>[2x]SNAMAIHNRAGQPAQQSDLINVAQLTAQYYVLKPEAGNAEHAVKFGTSGHRGSAGRHSFNEPHILAIAQAIAEERAKNGITGPCYVGKDTHALSEPAFISVLEVLAANGVDVIVQENNGFTPTPAVSNAILVHNKKGGPLADGIVITPSHNPPEDGGIKYNPPNGGPADTNVTKVVEDRANALLAGGLQGVKRISLDAAMASGHVKAVDLVQPFVEGLADIVDMAAIQKAGLTLG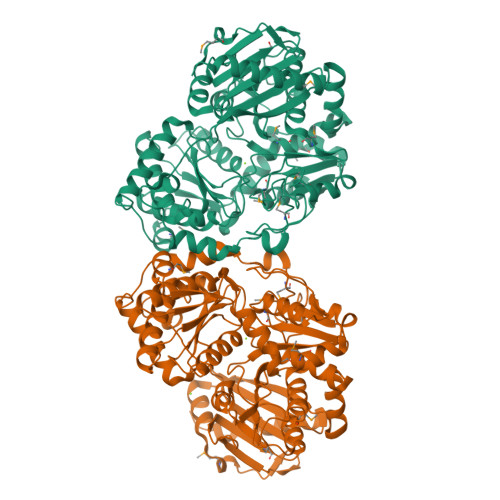VDPLGGSGIEYWKRIAEHYKLNLTLVNDQVDQTFRFMHLDKDGAIRMDCSSECAMAGLLALRDKFDLAFANDPDYDRHGIVTPAGLMNPNHYLAVAINYLFQHRPLWGKDVAVGKTLVSSAMIDRVVNDLGRKLVEVPVGFKWFVDGLFDGSFGFGGEESAGASFLRFDGTPWSTDKDGIIMCLLAAEITAVTGKNPQEHYNELAARFGAPSYNRLQASATSAQKAALSKLSPEMVSASTLAGDPITARLTAAPGNGASIGGLKVMTDNGWFAARPSGTEDAYKIYCESFLGEEHRKQIEKEAVEIVSEVLKNA> MHHHHHHTT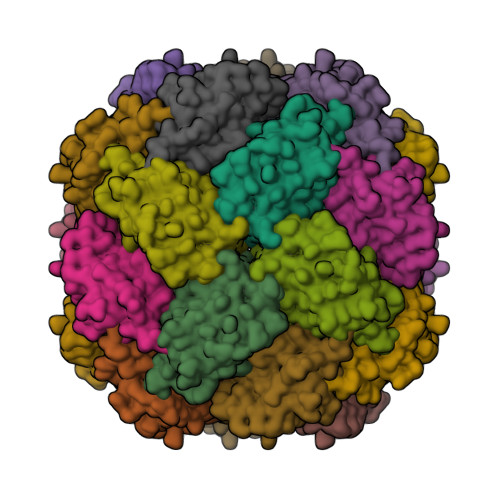TQTAKASRRARIERRTRESDIVIELDLDGTGQVAVDTGVPFYDHMLTALGSHASFDLTVRATGDVEIEAHHTIEDTAIALGTALGQALGDKRGIRRFGDAFIPMDETLAHAAVDLSGRPYCVHTGEPDHLQHTTIAGSSVPYHTVINRHVFESLAANARIALHVRVLYGRDPHHITEAQYKAVARALRQAVEPDPRVSGVPSTKGAL>MAYELPELPYAYDALEPHIDKET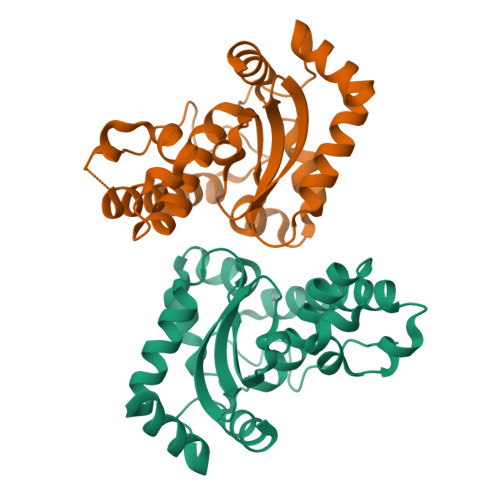MTIHHTKHHNTYVTNLNKAVEGNTALANKSVEELVADLDSVPENIRTAVRNNGGGHANHKLFWTLLSPNGGGEPTGALAEEINSVFGSFDKFKEQFAAAAAGRFGSGWAWLVVNNGKLEITSTPNQDSPLSEGKTPILGLDVWEHAYYLNYQNRRPDYISAFWNVVNWDEVARLYSERK[8x]> GGA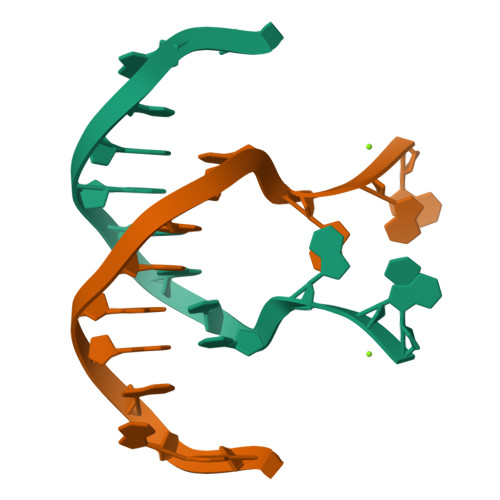CCATGGGGAG>[8x]METDLNSQDRKDLDKFIKFFALKTVQVI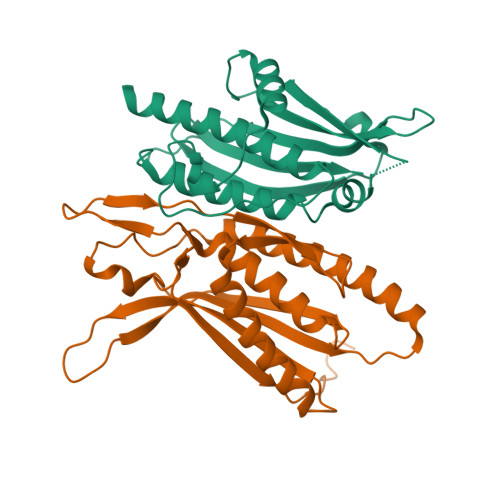VQARLGEKICTRSSSSPTGSDWFNLAIKDIPEVTHEAKKALAGQLPAVGRSMCVEISLKTSEGDSMELEIWCLEMNEKCDKEIKVSYTVYNRLSLLLKSLLAITRVTPAYRLSRKQGHEYVILYRIYFGEVQLSGLGEGFQTVRVGTVGTPVGTITLSCAYR;>MNCRSEVLEVSVEGRQVEEAMLAVLHTVLLHRSTGKFHYAAAGTYSIGTVGTQDVDCDFIDFTYVRVSSEELDRALRKVVGEFKDALRNSGGDGLGQMSLEFYQKKKSRWPFSDECIPWEVWTVKVHVVALATEQERQICREKVGEKLCEKIINIVEVMNRHEYLPKMPTQSEVDNVFDTGLRDVQPYLYKISFQITDALGTSVTTTMRRLIKDTLAL[8x]>SNVMFKKIKSFEVVFNDPEKVYGSGERVAGRVIVEVSEVTRVKAVRILASGVAKVLWMQGSQQCKQTSEYLRYEDTLLLEDQPTGENEMVIMRPGNKYEYKFGFELPQGPLGTSFKGKYGSVDYWVKAFLDRPSQPTQETKKNFEV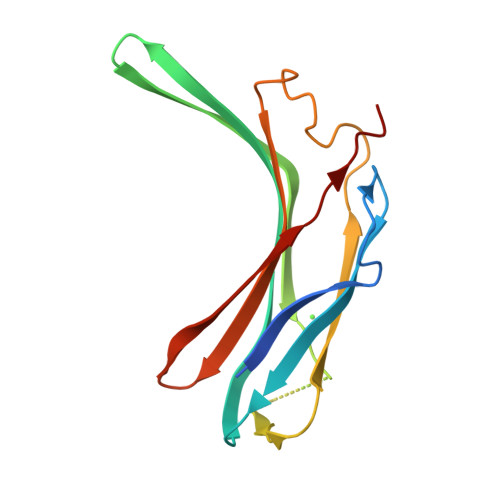VDLV[10x]>GHMNQFVTNTKNVIRGKYHPEFLQNEVLADIFAHTAQTLPDKTALIEADKTLSYGELYQQALIMAQHLALKGVKPGHIVGLWLPRGIELLKAQLAICLSGAAWLPFDMDTPADRIAVCLEDAEAVGMITTDEWYEHLAEVPQTKWTNTELQKPLSESVSLAKTTPDQPAYIIYTSGSTGKPKGIVITQKNICHFLRSENSILGIQEQDKVYQGFSVAFDMSFEEIWLSYLVGATLWIAPKSLVSDPERLCQTLKQEQITVLHAVPTLLALFPEDVPNLRIINLGGEMCPDSLVDRWALPHHQMFNTYGPTETTVSASLELLERGKPVTIGKPLPNYGMLVINSERELLEQGETGELCIFGPSVAQGYLGRPDLTADKFIENPWAMSVEEELLYRTGDLAKIDEFGQVHCLGRA[2x]

Here, we report a δ-poly-L-ornithine synthetase from Acinetobacter baumannii, which we name PosA. Nonribosomal peptide synthetase (NRPS) enzymes, usually composed of condensation, adenylation, and thiolation domains, are involved in peptide natural product biosynthesis to produce antibiotics and siderophores. Activity analyses show that the A. baumannii homolog activates L-Orn and the full-length protein produces isopeptide polymers in vitro. Structures of the isolated adenylation domain from PosA are presented with several diamino acids and biochemical assays identify important substrate binding residues.

To better understand the substrate binding in PosA, we solved four structures of the isolated adenylation domain. The α-amino groups of all three substrates, L-ornithine, D-ornithine, and L-lysine, interact with of Asp217 in co-crystal structures. Glu221 showed charged interaction with terminal δ-amine of ornithine substrates or the ε-amino group of lysine indicating an important role in binding. Density for both ornithine isomers was unambiguous; the electron density for the lysine ligand was less complete for the carboxylate and amine, suggesting the longer substrate may adopt multiple conformations in the active site of the crystallized protein. The adenylation domain showed modest activity with L-lysine and a reproducible low level of activity with L-arginine and L-histidine. Michaelis-Menton kinetics showed a preference in the apparent kcat/KM of over 160-fold for L-ornithine compared with L-lysine. As Met218 shows 3.9 Å hydrophobic interaction with Cδ of L-ornithine, it may play an important role in the specificity of substrates, since CHPAs adenylation domains activating Lys have an alanine and PDAP synthetase has a phenylalanine residue at the respective position of Met218 in PosA. However, the apparent kcat/KM increased nearly 10-fold for L-Lys for the M218A mutant. Structural modeling of M218A mutation showed an increased volume of cavity in the substrate binding pocket supporting the role of methionine as a steric hindrance for substrates longer than ornithine. The assays showed no peptide peak on SP cation exchange chromatography nor the presence of lysine polymers with LC/MS.>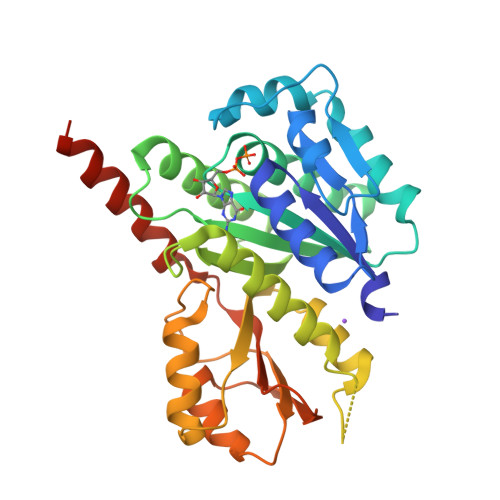 PHMKNKIVFAPIGQGGGNIVDTLLGICGDYNALFINTSKKDLDSLKHAKHTYHIPYAEGCGKERKKAVGYAQTYYKQIIAQIMEKFSSCDIVIFVATMAGGTGSGITPPILGLAKQMYPNKHFGFVGVLPKATEDIDEHMNAIACWNDIMRSTNEGKDISIYLLDNNKREKESDINKEFATLFNDFMNMSESHAEGVVDEDEISKLLTMKKSNVILEFDDKEDIQVALAKSLKESIFAEYTTNTCEFMGISTTRVVDVEAIKSIVGYPRRTFKGYNSKKNIVVATGIEPQKTTVQMMNEIIEDKMKQRREVTSKSENM> MSGSMKEEIKRL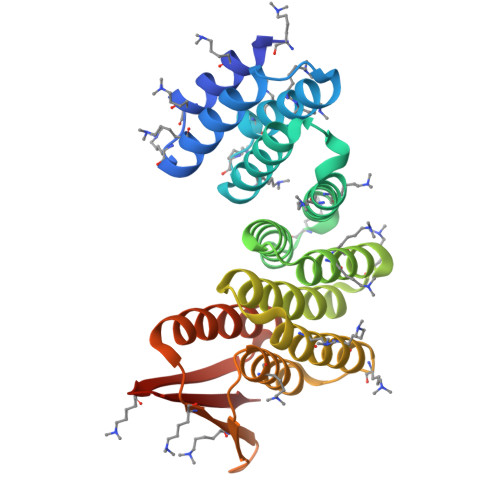AEELKEKTKNEEIKRLAEEAAELAERSDDPEVLEVVKKALEEALKSKNEEKIELLLLVAVLVAEAGSVDAVEEKLEIALLALKLAEESKDPRIIRGALRAAIAALRSDDPLALKTVKEALERARASKDERLIRAILAAAYAFALLAVAGASAERLKEAEAIVKELIAAAEKGASPQELVLLVIEMMVKGMGVTMETHRSGNEVKVVIKGLHESQQEVLLEAVLFAAELMGVRVRIRFKGDTVTIVVREGSG N-[(benzyloxy)carbonyl]-N-methyl-L-alanine 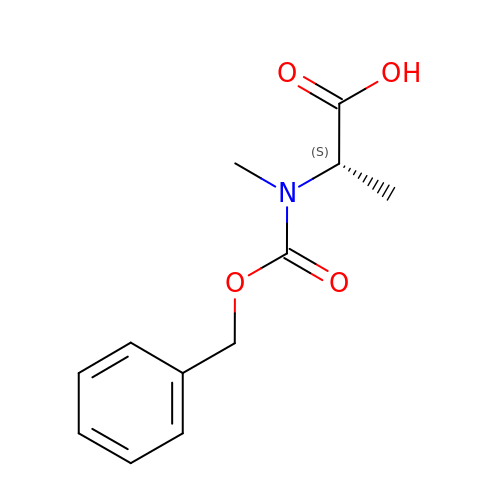| C12 H15 N O4 | QGEQKVZQPWSOTI-VIFPVBQESA-N> FADRMVIKAQSPAGFAEEYIIESIWNNRFPPGTILPAERELSELIGVTRTTLREVLQRLARDGWLTIQHGKPTKVNNFWETSGLNILETLARLDHESVPQLIDNLLSVRTNISTIFIRTAFRQHPDKAQEVLATANEVADHADAFAELDYN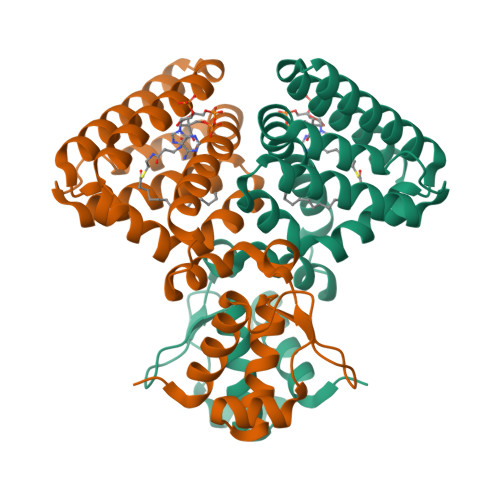IFRGLAFASGNPIYGLILNGMKGLYTRIGRHYFANPEARSLALGFYHKLSALCSEGAHDQVYETVRRYGHESGEIWHRMQKNLPGDLAIQGR> RSPWPPYKSSGIYEEEPQLPGASDLSGGVASDEIGVAPAQAVDERYRLPTTSIPIHYDLHLRTEIHRNERTFTGTVGIQLQVVQATDKLVMHNRGLVMSSAKVSSLPNGVTGAPTLIGDVQYSTDTTFEHITFTSPTILQPGTYLLEVAFQGRLATNDDGFYVSSYVADNGERRYLATTQFESTSARMAFPCYDEPGLKATFTVSITHSLSYKAISNMPQKTTTDIETDMRTTFFEKTPAMSTYLLAFVVSDFQLRLSGAQRVYVRPNAFNEATFALEAGVKILKVLDDHLGIPYDTYMPKLDQIAIPDFAAGAMENWGLVTYREQALLFNPAVSTYRGKTNVATTIAHEYAHQWFGNLVSPEWWEYIWLNEGFATLYEFYALDMAYPGQEYWELFNQQVIQYAMGQDGQASTRPMNWNAATPGEISALFDRVAYDKSGSVLNMMRHVLGDDNWKAGLKAY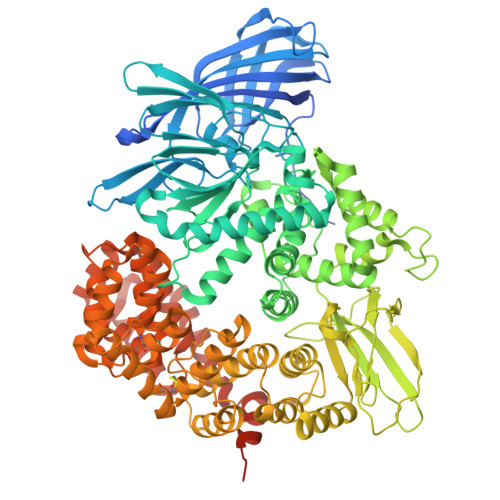LTDRALQGAVDEQLYAGLQSAIEGKGVLPNGVTVAQIMRTWTNEAGYPVLNVRRSYDTGDVIISQERFYNDRKVPNTNIWMIPYNYVHQAKADFNEFDDFQWLATKAARIETTVPANEWIVFNKQQVGYYRVNYDEHNWELITNALHENWASIHRLNRAQLIDDAYWLARSGRLDLRVALRFMTYLRNEREYAPWTAANVALTYFNNRLRGTAEYHNFLIFVDALIEDIYSLLTIDAVSPDDTLLHKYLVQTISTWACSMGYTDCLMKTAALLKAEASGTGPAVHPDIASVTYCYGMRSALESEFQYLYRKMMNSKNLAERTMLIDSLGCSNNKEFLKAFLTTALGSGTGVEINYRADERRRVVQAIYSGGRTGVDALIEFLMDPALVNEFVSTLSTSTLNSALSAIASRTNNVEEMNKLNALITALGSRVNSQTAANLRTTAQANLDWVNGFEGLMLSNFLAEAAARGHPFEGKPIPNPLLGLDSTRTGHHHHHH> MSEPMMWLLVRGVWETLAMTFVSGFFGFVI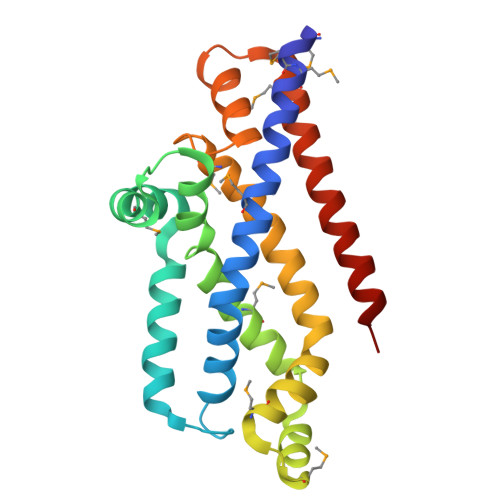GLPVGVLLYVTRPGQIIANAKLYRTVSAIVNIFRSIPFIILLVWMIPFTRVIVGTSIGLQAAIVPLTVGAAPFIARMVENALLEIPTGLIEASRAMGATPMQIVRKVLLPEALPGLVNAATITLITLVGYSAMGGAVGAGGLGQIGYQYGYIGYNATVMNTVLVLLVILVYLIQFAGDRIVRAVTRK>[2x]MTNSTDGRAD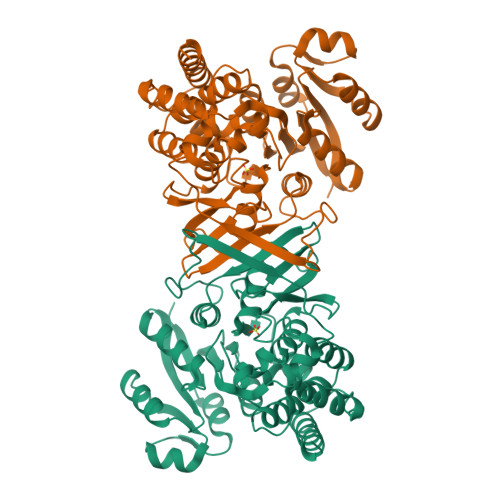GRLRVVVLGSTGSIGTQALQVIADNPDRFEVVGLAAGGAHLDTLLRQRAQTGVTNIAVADEHAAQRVGDIPYHGSDAATRLVEQTEADVVLNALVGALGLRPTLAALKTGARLALANKESLVAGGSLVLRAARPGQIVPVDSEHSALAQCLRGGTPDEVAKLVLTASGGPFRGWSAADLEHVTPEQAGAHPTWSMGPMNTLNSASLVNKGLEVIETHLLFGIPYDRIDVVVHPQSIIHSMVTFIDGSTIAQASPPDMKLPISLALGWPRRVSGAAAACDFHTASSWEFEPLDTDVFPAVELARQAGVAGGCMTAVYNAANEEAAAAFLAGRIGFPAIVGIIADVLHAADQWAVEPATVDDVLDAQRWARERAQRAVSGMASVAIASTAKPGAAGRHASTLERS> GAMEATPTPADLFSEDYLVDTLDGLTVDDQQAVLASLSFSKFLKHAKVRDWCAQAKIQPSMPALRMAYNYFLFSKVGEFIGSEDVCNFFVDRVFGGVRLLDVASVYAACSQMNAHQRHHICCLVERATSSQSLNPVWDALRDGIISSSKFHWAVKQQNTSKKIFSPWPITNNHFVAGPL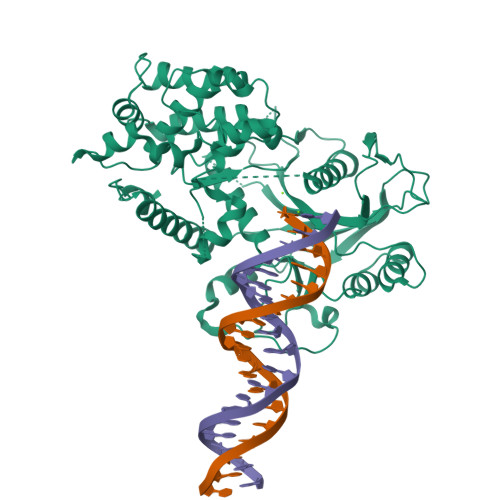AFGLRCEEVVKTLLATLLHPDETNCLDYGFMQSPQNGIFGVSLDFAANVKTDTEGRLQFDPNCKVYEIKCRFKYTFAKMECDPIYAAYQRLYEAPGKLALKDFFYSISKPAVEYVGLGKLPSESDYLVAYDQEWEACPRKKRKLTPLHNLIRECILHNSTTESDVYVLTDPQDTRGQISIKARFKANLFVNVRHSYFYQVLLQSSIVEEYIGLDSGIPRLGSPKYYIATGFFRKRGYQDPVNCTIGGDALDPHVEIPTLLIVTPVYFPRGAKHRLLHQAANFWSRSAKDTFPYIKWDFSYLSANVPHSP>[2x]MGSDKIHHHHHHMKITWFGHACFALEMEGKTIVTDPFDESVGYPIPNVTADVVTESHQHFDHNAHHLVKGNFRVIDRPGAYTVNGVKIKGVETFHDPSHGRERGKNIVFV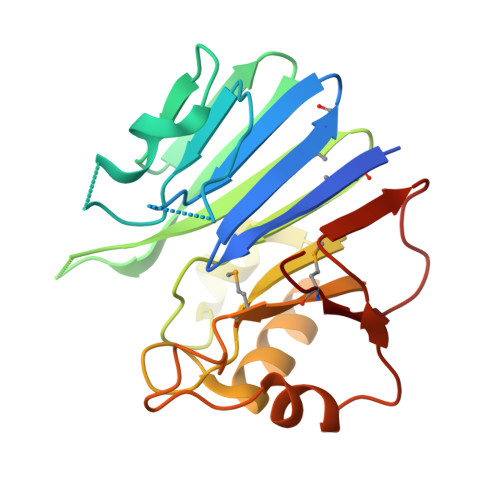FEGEGIKVCHLGDLGHVLTPAQVEEIGEIDVLLVPVGGTYTIGPKEAKEVADLLNAKVIIPMHYKTKYLKFNLLPVDDFLKLFDSYERVGNILELFEKPKERKVVVMEVQ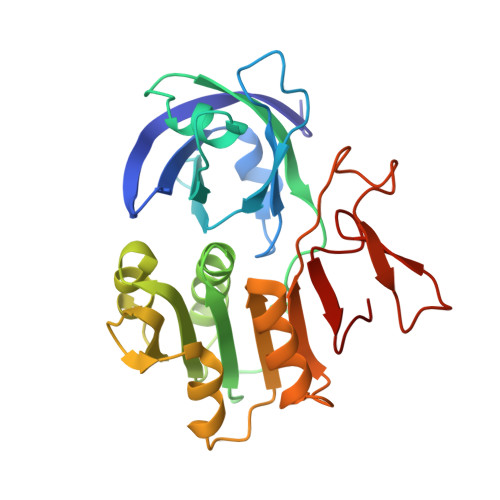> SQLQEMMTVVSQREVAYNIFEMVLKGTLVDEMDLPGQFLHLAVPNGAMLLRRPISISSWDKRAKTCTILYRIGDETTGTYKLSKLESGAKVDVMGPLGNGFPVAEVTSTDKILIIGGGIGVPPLYELAKQLEKTGCQMTILLGFASENVKILENEFSNLKNVTLKIATDDGSYGTKGHVGMLMNEIDFEVDALYTCGAPAMLKAVAKKYDQLERLYISMESRMACGIGACYACVEHDKEDESHALKVCEDGPVFLGKQLSL> GHMSQIPASEQETLVRPKPLLLKLLKSVGAQKDTYT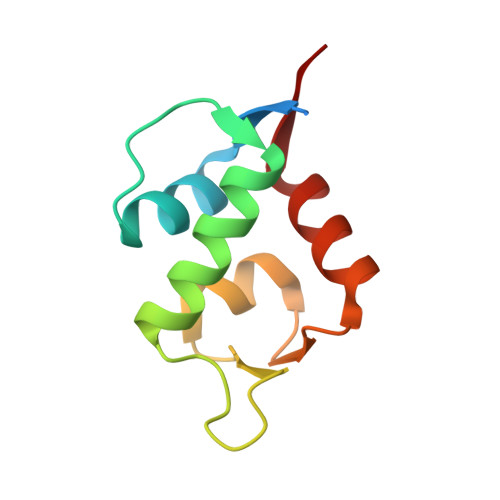MKEVLFYLGQYIMTKRLYDEKQQHIVYCSNDLLGDLFGAPSFSVKEHRKIYTMIYRNLVVVN A third vital component of the TFP biogenesis system is the assembly ATPase (PilF in T. thermophilus). The TFP assembly ATPases are part of the extensive AAA+ superfamily which form molecular motors, using the energy from ATP hydrolysis to drive mechanical transformations. The domain structure of T2SS and TFP biogenesis ATPases is similar, in that they comprise one or more N1 or GSPII domains at the N-terminus, followed by a C-terminal (CTD) and N2 domain- which comprise the ATP binding site. Here we present a combination of X-ray crystallographic and cryoelectron microscopy single particle reconstructions of the PilF hexamer in two states which are used to build molecular models for the complete PilF hexamer and chart its structural transition on binding of ATP.

The fit of the docked model was optimized by refinement in ROSETTA27, giving the model TtPilFAMPPNP. The TtPilFAMPPNP structure was then used as a starting point for refinement against the apoprotein map, and the final model was designated TtPilFapo; structures of both forms are shown in Fig. 3. Of particular note is the fact that the part of the structure associated with the ATPase domains is more distorted from C6 symmetry than the N1 domain section. A comparison of the two density maps revealed that they are similar in overall shape and dimensions, but the apoprotein structure is shorter and wider than the AMPPNP structure, indicative of conformational change between the two states (discussed further below). The apoprotein structure showed a consistent contraction towards the center of the complex for all domains- readily apparent from a superposition of both structures and also an analysis of the displacement of the centers of mass. Displacement of the N2 domains appeared to be generally greater than the CTDs: this observation is significant because it is this domain which is linked to the N1 domains in the N-terminal half of TtPilF. It therefore appears that binding of AMPPNP to TtPilFapo triggers an expansion of the hexamer, outwards from the center. We conclude, therefore, that the transition from TtPilFapo to TtPilFAMPPNP is better described by an outward shift in center of mass, particularly of the N2 domains, rather than changes in the relative orientation of adjacent CTD/N2 units. Calculations of centers of mass for each domain showed that the TtPilFAMPPNP N1 domains from both ring 1 and ring 2 are displaced downwards by distances of 4–9 Å. This is accompanied by rotation outwards (mean value 14o for ring 2 domains), which leads to a wider aperture at the base of the structure. Combined, these movements lead to changes in the relative positions of the N1 domains in ring 2 of 10–13 Å which occur on the transition from TtPilFAMPPNP to TtPilFapo and therefore, by implication, after hydrolysis of ATP.

>[6x]SAAQKFVKQVIREAFLQDASDIHIEPRQNDVQVRLRIDGALRPYSTLPKGALNAVISVVKIMGGLNIAEKRLPQDGRVRYREGAIDVDLRLSTLPTVYGEKAVMRLLKKASDIPEIEDLGFAPGVFERFKEVISKPYGIFLITGPTGSGKSFTTFSILKRIATPDKNTQTIEDPVEYEIPGINQTQVNPQAGLTFARALRAFLRQDPDIIMVGEIRDSETAKIATEAALTGHLVIATLHTNDAAQAITRLDEMGVEPFNISAALIGVLSQRLVRRVCEHCKVEVKPDPETLRRLGLSEAEIQGARLYKGMGCERCGGTGYKGRYAIHELLVVDDEIRHAIVAGKSATEIKEIARRKGMKTLREDGLYKALQGITTLEEVLARTIEAAAELALVPRGSSAHHHHHHHHHH;>[6x]LPRAKPLGEILVELGLARPEDVEEALQKQRRGGGRLEDTLVQSGKLRPEALAQAVATQLGYPYVDPEEDPPDPGAPLLLPEDLCRRYGVFPHRLEGNRLVLLMKDPRNILALDDVRLALKRKGLNYEVAPAVATEAAITKLIERFY;>QKDLKLGELLLQKGWISREALEEALVEQEKTGDLLGRILVRKGLPEEALYRALAEQKGLEFLESTEGIVPDPSAALLLLRSDALRYGAVPIGFQNGEVEVVLSDPRHKEAVAQLLNRPARFYLALPQAWEELFRRAY[6x]>[2x]SNAKSPQDMDRFIDALMKKMTVEEKIGQLNLPVSGEIVTGQAQNSDVAKKIEQGLVGGLLNLKGVEKIRDVQKLAIEKSRLGIPLIFGMDVVHGYETIFPIPLGLSCSWDMEAIRKSARVAAIEASADGISWTFSPMVDISRDPRWGRVSEGNGEDPFLGGAIAKAMVSGYQGIDLNNQLKRNDEIMACVKHFALYGAGEAGRDYNTVDMSRNRMFNEYMYPYQAAVDAGVGSVMASFNEIDGIPATANKWLMTDVLRKQWGFDGFVVTDFTGISEMIAHGIGDLQTVSARALNAGVDMDMVSEGFTGTIKKSIDEGKISMETLDKACRRILEAKYKLG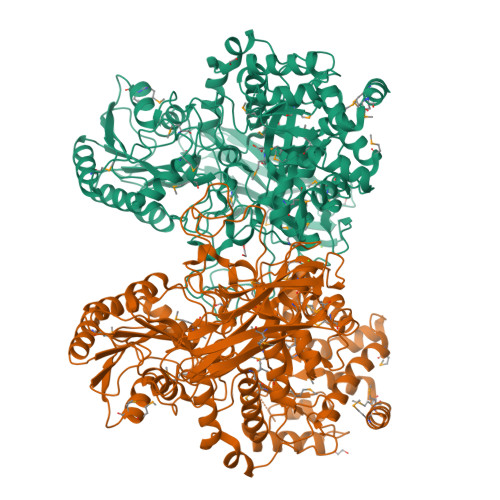LFDNPYKYCDLKRPKRDIFTKEHRDAARKIAGESFVLLKNDKSGSSANPTLPLKKEGTVAVIGPLANTRSNMPGTWSVAARLNDYPSVYEGLKEMMKGKVNITYAKGSNLISDAAYEERATMFGRSLNRDNRTDKEMLDEALKVAANADVIIAALGESSEMSGESSSRTNLALPDVQRTLLEALLKTGKPVVLTLFTGRPLTLTWEQEHVPAILNVWFGGSEAAYAIGDVLFGDVNPSGKLTMTFPKNVGQIPLFYNHKNTGRPLLEGKWFEKFRSNYLDVDNDPLYPFGYGLSYTNFQYSDITLSAPTMGQDGSVTAMVTVTNTGKYDGAEVVQLYIRDLVGSITRPVKELKGFDKIFLKAGESKTVSFKITPELLRFYDYELNYVAEPGDFDIMIGGNSQSVKTTHLSLK>XSKLLELLRKLGEALHK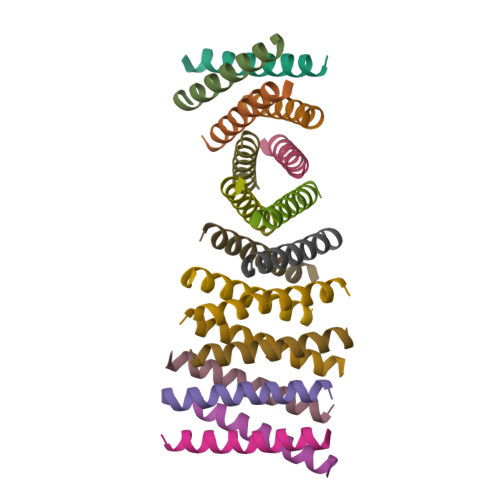AIELLEKWGX[18x]> MVLLESEQFLTELTRLFQKCRTSGS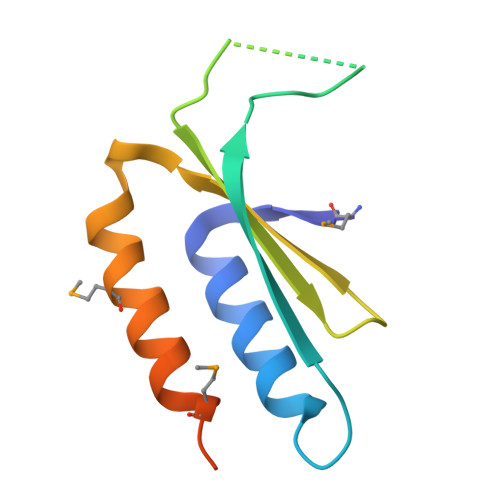VYITLKKYDGRTKPIPKKGTVEGFEPADNKCLLRATDGKKKISTVVSSKEVNKFQMAYSNLLRANMDGLKKRDKKNKTKKTK> HMSSGSAGLSSLHRTYSQDCSFKNSMYHVGDYVYVEPAEANLQPHIVCIERLWEDSAGEKWLYGCWFYRPNETFHLATRKFLEKEVFKSDYYNKVPVSKILGKCVVMFVKEYFKLCPENFRDEDVYVCE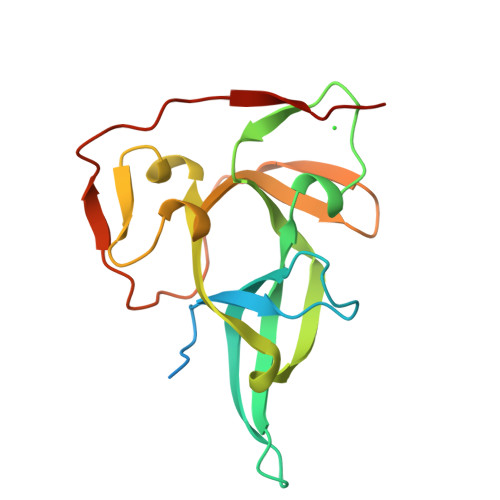SRYSAKTKSFKKIKLWTMPVSSVRFVPRDVPLPVVRVASVFANTD Influenza virus genome encapsidation is essential for the formation of a helical viral ribonucleoprotein (vRNP) complex composed of nucleoproteins (NP), the trimeric polymerase, and the viral genome. Within each vRNP, the viral RNA (vRNA) segment is encapsidated by the viral nucleoprotein (NP) and attached to the heterotrimeric RNA-dependent RNA polymerase. In this study, we established a biological tool, the RNP-like particles assembled from recombinant influenza A virus NP and synthetic RNA, and we present the first subnanometric cryo–electron microscopy structure of the helical NP-RNA complex (8.7 to 5.3 Å). The RNP-like particles are a tool that mimics the influenza nucleocapsid.

Therefore, we performed a local refinement focused on three successive NP protomers along the same strand (called later in the text NP−1, NP, and NP+1, respectively) (boxed region, and C). The small RNA molecule is located at the interface between two NP protomers. Of note, the RNA density local resolution varies between 4.5 and 6.8 Å, suggesting that the RNA is globally dynamic within the RNP-like structure; therefore, we only modeled the phospho-ribose chain, and we did not assess the direction (5′ to 3′) of the RNA structure. Here, we observe that residues R150, R152, R156, R355, and R361 most likely interact with the RNA phosphate backbone and that Y148 and F458 may interact with the RNA bases, while residues Q149, K273, and R391 are in the close vicinity of the RNA and could also be involved in its binding. Observation of our structure indicates that an RNA molecule of at least 10 nt is required to bridge the NPs together at the NP-NP interface and thus to form the RNP helical architecture. With this modeling, about 22 to 24 nt can be fitted per NP protomer (12 nt buried at the NP-NP interface and about 10 to 12 nt across the central basic groove), agreeing with the previous studies establishing the RNA (24 nt) for one NP stoichiometry using mass spectrometry and biochemistry coupled with EM. The overall structures are similar, except for the oligomerization loop (residues 402 to 428), which displays considerable flexibility and various orientations, as well as a loop spanning residues D72 to K90, which also revealed several conformations and notably an α helix in our structure. In addition, upon RNA binding, the flexible D72-K90 loop folds into an α helix, increasing the accessibility of the central basic groove.

>[3x]MATKGTKRSYEQMETDGERQNATEIRASVGKMIDGIGRFYIQMCTELKLSDYEGRLIQNSLTIERMVLSAFDERRNKYLEEHPSAGKDPKKTGGPIYRRVDGKWRRELILYDKEEIRRIWRQANNGDDATAGLTHMMIWHSNLNDATYQRTRALVRTGMDPRMCSLMQGSTLPRRSGAAGAAVKGVGTMVMELIRMIKRGINDRNFWRGENGRRTRIAYERMCNILKGKFQTAAQRTMVDQVRESRNPGNAEFEDLIFLARSALILRGSVAHKSCLPACVYGSAVASGYDFEREGYSLVGIDPFRLLQNSQVYSLIRPNENPAHKSQLVWMACHSAAFEDLRVSSFIRGTKVVPRGKLSTRGVQIASNENMETMESSTLELRSRYWAIRTRSGGNTNQQRASSGQISIQPTFSVQRNLPFDRPTIMAAFTGNTEGRTSDMRTEIIRLMESARPEDVSFQGRGVFELSDEKATSPIVPSFDMSNEGSYFFGDNAEEYDNLEHHHHHH>GCGTATACGC[2x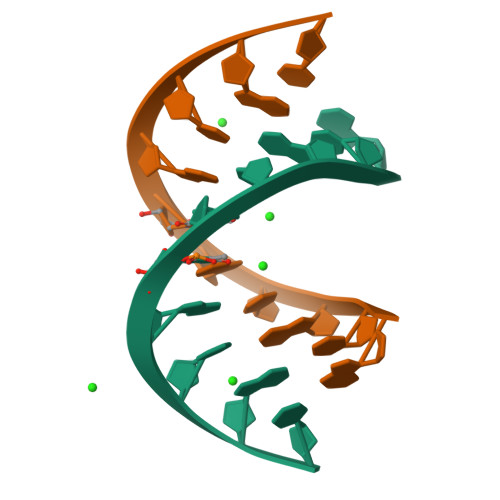]> SDNAIAMEAAHSKSTEECLAYFGVSETTGLTPDQVKRHLEKYGHNELPAEEGKSLWELVIEQFEDLLVRILLLAACISFVLAWFEEGEETITAFVEPFVILLILIANAIVGVWQERNAENAIEALKEYEPEMGKVYRADRKSVQRIKARDIVPGDIVEVAVGDKVPADIRILSIKSTTLRVDQSILTGESVSV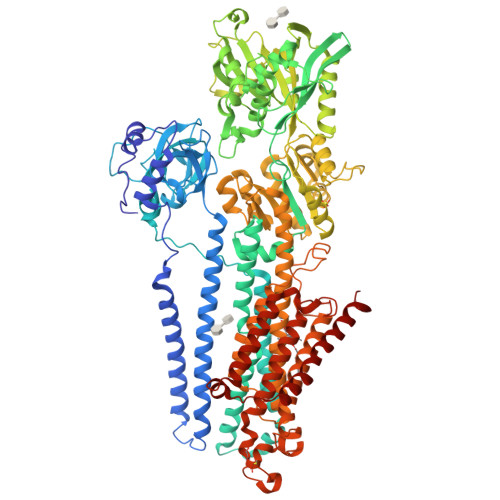IKHTEPVPDPRAVNQDKKNMLFSGTNIAAGKALGIVATTGVSTEIGKIRDQMAATEQDKTPLQQKLDEFGEQLSKVISLICVAVWLINIGHFNDPVHGGSWIRGAIYYFKIAVALAVAAIPQGLPAVITTCLALGTRRMAKKNAIVRSLPSVETLGCTSVICSDKTGTLTTNQMSVCKMFIIDKVDGDFCSLNEFSITGSTYAPEGEVLKNDKPIRSGQFDGLVELATICALCNDSSLDFNETKGVYEKVGEATETALTTLVEKMNVFNTEVRNLSKVERANACNSVIRQLMKKEFTLEFSRDRKSMSVYCSPAKSSRAAVGNKMFVKGAPEGVIDRCNYVRVGTTRVPMTGPVKEKILSVIKEWGTGRDTLRCLALATRDTPPKREEMVLDDSSRFMEYETDLTFVGVVGMLDPPRKEVMGSIQLCRDAGIRVIMITGDNKGTAIAICRRIGIFGENEEVADRAYTGREFDDLPLAEQREACRRACCFARVEPSHKSKIVEYLQSYDEITAMTGDGVNDAPALKKAEIGIAMGSGTAVAKTASEMVLADDNFSTIVAAVEEGRAIYNNMKQFIRYLISSNVGEVVCIFLTAALGLPEALIPVQLLWVNLVTDGLPATALGFNPPDLDIMDRPPRSPKEPLISGWLFFRYMAIGGYVGAATVGAAAWWFMYAEDGPGVTYHQLTHFMQCTEDHPHFEGLDCEIFEAPEPMTMALSVLVTIEMCNALNSLSENQSLMRMPPWVNIWLLGSICLSMSLHFLILYVDPLPMIFKLKALDLTQWLMVLKISLPVIGLDEILKFIARNYLEG Eukaryotic mitochondrial RNA splicing 2 (Mrs2), a homolog of prokaryotic CorA, anchors to the inner mitochondrial membrane and mediates the influx of Mg2+ into the mitochondrial matrix. The overall structure of the hMrs2 channel has a cone shape, and it is assembled into a pentamer with a central pore in the middle. The pentameric hMrs2 structure can be further separated into two parts: the N-terminal funnel domain within the matrix and the C-terminal transmembrane domain in the inner mitochondrial membrane. Molecular dynamics simulations and mitochondrial Mg2+ uptake assays show that the R-ring may function as a charge repulsion barrier, and Cl− may function as a ferry to jointly gate Mg2+ permeation in hMrs2.

The hMrs2 structure was reconstructed from the dataset in the presence of 20 mM Mg2+, pH 8.0 (hereinafter referred to as hMrs2-Mg); from the dataset without the addition of external Mg2+ or EDTA, pH 8.0 (named hMrs2-rest); from the dataset in the presence of 1 mM EDTA, pH 8.0 (named hMrs2-lowEDTA); or from the dataset in the presence of 5 mM EDTA, pH 6.8 (named hMrs2-highEDTA). In the hMrs2-Mg structure, four Mg2+-binding sites and one Cl−-binding site were identified. The first Mg2+-binding site (called Mg-1) is located inside the pore mouth on the intermembrane side. The second Mg2+-binding site (called Mg-2) is located in the pentameric center of the matrix part of the hMrs2 channel, positioned immediately below the inner leaflet of the membrane. The third Mg2+-binding site (called Mg-3) is located in the middle high region of the hMrs2 matrix part within the interface between two adjacent protomers. Mg2+ is coordinated by three carboxylic acid residues (E138, E243 and D247) in one protomer and one carboxylic acid group of residue E312 in another protomer. The fourth Mg2+-binding site (called Mg-4) is located in the near bottom region of hMrs2 within the interface between two protomers. Mg2+ is coordinated at this site by two carboxylic acid residues (E297 and E293) in one protomer and one carboxylic acid group of residue E261 in another protomer. The Cl−-binding site (called Cl-1) is located in the pentameric center of the transmembrane part of the hMrs2 channel, very close to the inner leaflet of the membrane. Of the five ligand-binding sites, three sites (Mg-1, Mg-2 and Cl-1) but not the other two binding sites (Mg-3 and Mg-4) are located in the three other aforementioned hMrs2 structures (hMrs2-rest, hMrs2-lowEDTA and hMrs2-highEDTA).

>[5x]MECLRSLPCLLPRAMRLPRRTLCALALDVTSVGPPVAACGRRANLIGRSRAAQLCGPDRLRVAGEVHRFRTSDVSQATLASVAPVFTVTKFDKQGNVTSFERKKTELYQELGLQARDLRFQHVMSITVRNNRIIMRMEYLKAVITPECLLILDYRNLNLEQWLFRELPSQLSGEGQLVTYPLPFEFRAIEALLQYWINTLQGKLSILQPLILETLDALVDPKHSSVDRSKLHILLQNGKSLSELETDIKIFKESILEILDEEELLEELCVSKWSDPQVFEKSSAGIDHAEEMELLLENYYRLADDLSNAARELRVLIDDSQSIIFINLDSHRNVMMRLNLQLTMGTFSLSLFGLMGVAFGMNLESSLEEDHRIFWLITGIMFMGSGLIWRRLLSFLGRQLEAPLPPMMASLPKKTLLADRSMELKNSLRLDGLGSGRSILTNRSADYKDDDDK>[2x]MGSSHHHHHHENLYFQSNAETVAAIKTLIQQLAQSTDQFGRAEINDALRELQYSLETPFDTVMRMSLDTAQVAVARIGSDLGLFKHLSQCASPQSAEELADHLGCGRELMSRLLRYMASVRMVQQTDDIKYISSNITQTLAVPGLEAGMRHAFENLWPVLMALPDFLAERKYPDIVDAKD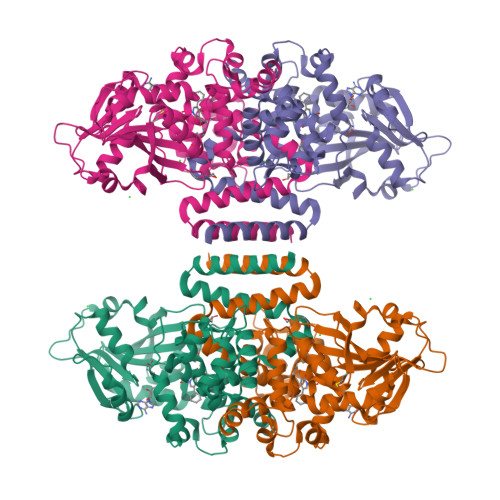TAFQKAFNTDQDCFHWLATQPTRIANFKVLLTDERTPNFLSTFPLEKELGSWSAEPEKALFVDIGGGMGHACIRLREKYPNQPGRVILQDLPPVLQAAQATLPLSGIESMPHNFHTPQPVQGAKFYFLRLILRDFPDHQALEILQNIVPAMDAESRIVIDDGVPPEKGARWAETGTDICIMSALGSKERTQRQWEELAAKAGLQLQALYQYTWPVVNAAMVFSLQ> GPGSMLNTFMFPGQGSQAKGMGGALFDRFADLTAQADAVLGYSIRALCVDDPRDELGRTQFTQPALYVVNALTYYAKCEDSGETPDFLAGHSLGEFNALLAAGCFDFETGLKLVARRAELMS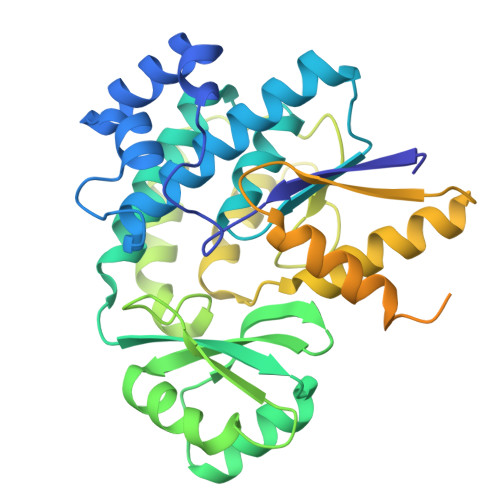QARDGAMAAIVNASREQIERTLDEHGLVDTAIANDNTPSQLVISGPAHEIARAEALFQHDRVRYLRLNTSGAFHSKFMRPAQQAFAAHLQSFRLADPAIPVISNVSARPYENGRVSEGLAQQIASPVRWCESIRYLLALAAERGEAIEFTELGHGDVLTRLVHTIRRQTPAPAAAATSARARPTPPGEPERPAQQTAAAPRASDSASASLGAAERVAAWNRDYPVGTRVRSSLIHDDVLETRTPATVLFGHRAAVYMKGYNGYFDLAEVTPA The S-adenosyl-L-methionine-dependent tRNA 4-demethylwyosine synthase TYW1 catalyzes biosynthesis of 4-demethylwyosine (imG-14), the precursor for wyosine, the hypermodified guanine-derived nucleotide present at position 37 of phenylalanine tRNAs of archaea and eukarya. Eukaryotic TYW1 enzymes contain N-terminal flavodoxin-like and C-terminal radical-SAM domains.

We determined co-crystal structures of the flavodoxin-like domain of the putative Tyw1 from Schizosaccharomyces japonicus in complex with flavin mononucleotide (FMN), exploiting an unexpected anomalous scatterer present in the recombinant protein. Our results show how eukaryotic TYW1 enzymes bind the coenzyme FMN and will help further elucidation of the structural enzymology of 4-demethylwyosine synthesis.

> KKLAKPEKIASATSLKGSTPKAPKVFRKTEKTKHSNRKIACEASTKSSRKLTDISACSINIFYSTLGGSTQKFAEHVADRIRSSLQTELVEILNLDYIDLDEYFSKGNSNTVYLVLLPSYAIESSIDYFLSALQTTIDDFRIVARPLEKLRGFAVLGFGDFEQYAGDLFCYQAIAADQRLAKLGAQRIAPLGVVNVKLEKAQVYEAMEAWTDLFLQYAKEKA>[2x]MQKVHVQYIDGETDQMLRQDDLDGYTDE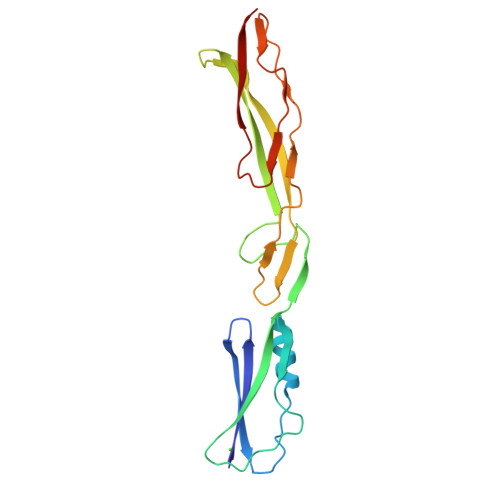TIPYSTAEGIKKFEGDGYELFKDNFPAGEKFDNDDTNDQFYTVIFKHHRENVDPNHSSADGTKGTKTLTETVHYKYANGTKAAEDQTAQVTFTRNGVLDDVTGIVAWGKWNEASQSYKALTSPTIAGYAPSEAVVKRSSNSDAEQGPTLTVIYTADA>[2x]MKHPFSRLFSFGEKEQEEMEEKQEREEVRHIPVKSIIPNRFQPRTMFDEEKIDELALTIRTHGIIQPIVVRECGNGRFEIIAGERRWRAVQKLGWTEIPAIIKNLNDKETASVALIENLQREELTPIEEAMAYAKLIELHDLTQEALAQRLGKGQSTIANKLRLLKLPQEVQEALLQRAITERHARALIALKDKEKQLKLLQEIIDKQLNVKQTEDRVLKLLEAGERKPKPKRKAFSRDKLAAALEHHHHHH

Here, we report that a nucleoid occlusion protein Noc is a CTPase enzyme whose membrane-binding activity is directly regulated by a CTP switch. In Bacillus subtilis, Noc nucleates on 16 bp NBS sites before associating with neighboring non-specific DNA to form large membrane-associated nucleoprotein complexes to physically occlude assembly of the cell division machinery. Unusually, Noc is also a peripheral membrane protein that directly associates with the cell membrane via a predicted N-terminal amphipathic helix (Adams et al., 2015). We provide evidence that (1) CTP is required for Noc to form the NBS-dependent nucleoprotein complex, and (2) CTP binding switches Noc from a membrane-inactive auto-repressed state to a membrane-active state.

However, we could grow and collect diffraction data for a C-terminal domain truncated apo-Noc (NocΔCTD) from a thermophilic bacterium, Geobacillus thermoleovorans, to 2.5 Å resolution. The structure was solved by iodide SAD phasing, as no other Noc protein family structure was available as a template for molecular replacement. The asymmetric unit contains two similar copies of monomeric apo-Noc (root-mean-square deviation [RMSD] = 0.9 Å), hence we used the more complete subunit for all further analysis. Each NocΔCTD subunit contains an NTD (helices α1–α6) and an NBS-specific DNA-binding domain (DBD) (helices α7–α12) (Jalal et al., 2020b; Wu et al., 2009). The primary dimerization domain at the C-terminal side of Noc was truncated in the NocΔCTD and hence was not present in this structure. Most notably, electron density for five of the 10 AA comprising the membrane-targeting helix α1 were visible in a 310 helical conformation. From the structure, it is apparent that the visible membrane-targeting sequence (AA 5–10) of Noc is indeed amphipathic, with distinct polar and hydrophobic faces. We noted that the hydrophobic face of the amphipathic α1 helix is buried toward α5 and α7 at the core of Noc and thus is unexposed and unlikely to be available for membrane interaction. Sidechains of F9 and F11 also interact hydrophobically with the side chains of I116 and I81, respectively. These interactions thus bury α1 in a potential autoinhibitory conformation.>TSHMGIRITGTGLFHPTEIISNEELADSLNAYVEQYNQENAEKIAAGELEELRGSSAEFIEKASGIKRRYVIEKSGILDPTRLRPRLSERSND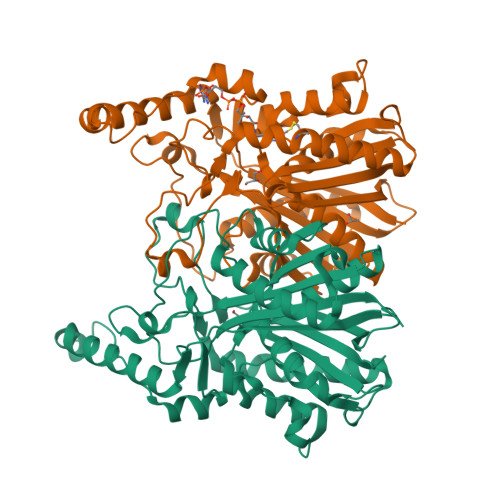ELSIQAEWGVIAAKQAMENAGVTAEDIDVVILACSNMQRAYPAVAIEIQSALGIQGYAYDMNVAASAATFGLKQAADAIRSGARRVLLVNVEITSGHLDYRNRDCHFIFGDVATASIIEETTTKTGFEILDIHLFTQFSNNIRNNFGFLNRSEDAVVDDKLFRQDGRKVFKDVCPLVAKIINAQLEKMQLTANDIKRFWLHQANANMNELILKYVAGKDADLSRAPIILDEFANTSSAGVIIALHRTGHEVDDGEYGVISSFGAGYSVGSIVVQKHVA[2x]>[2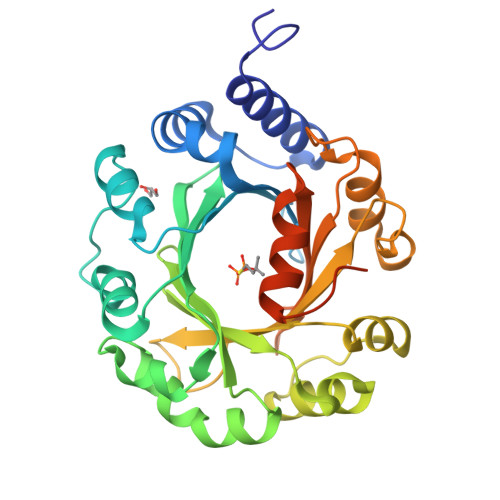x]GSAGAGAMTIVNRIRTDVVNVAKSFGAEYSEAVIDQIFQGFGEKFTNTGFAIRVQNKRNQKVDCNIRYGEAKENCLAWDIARESGLLSDQGHPVDTLIQEMFQAIPAIAYGADFDINYGLVKIWHLPKIVPVEEAFKIPSLPKSVNAHIDFFKKYHLDALCALTVDYRNKSTNLYFDAHHPEQRTTQFYKNILQSQQFEVPSDEVLEILVNCPEIAVTFNWSSPGIERMCFYTAFVNRETVPQHINPVLKKFAQEAPALLDNPGFLVGWSFGPDAKKGTYIKIDVDYHGLVVPSFFHMHNLPLPIPEANSVFDLPSSDTEDKLNSIVMS>[4x]MASTSVSPKTRETEAEAKAKKLDQKRLDEHEEEVRAREQQVRRPWHREGADKPPVEGNADPIAKGKLLTTPTRLLKLILPLPLRVEKDQKNNGRNNEYGRSISLNSDIQPLALLIHPQQPLSYVERLIQAELPPVVENGQEKIPNVYFRAEDSEQGDQKPTSRAEARSKDDGGEPSEYNTNLSHVAS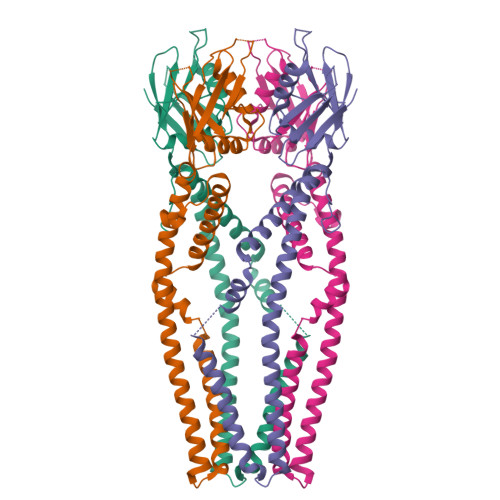ASGLGHRGPKRSSQDKRWVRWSSSTEMGDFIRDAARGREFAIEIEGYNIEMRVSVPSFGDRTYYMRQRLRKMSSEIDGLAKIKHECDLLAHRSAHRLAKGGFGLLAGWWGVVYYVTFHTEFGWDLVEPVTYLAGLTTIMGGYLWFLYINKDLSYKAAMNVTVSRRQHALYEMKGFDIERWEQLVQDANALRREIRVIAVEYDVDWDETRDVGEDVKDVLDEERSRRDDEHRSIEKEKDEKFTEDEKRKRKKDKESKETSGDSTNSHHHHHH> HMSQSNRELVVDFLSYKLSQKGYSWSQFSDVEENRTEAPEETEAERETPSAINGNPSWHLADSPAVNGATGHSSSLDAREVIPMAAVKQALREAGDEFELRARRAFSDLTSQ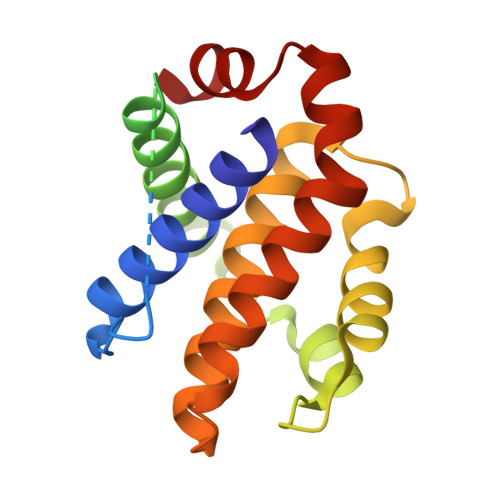LHITPGTAYQSFEQVVNELFRDGVNWGRIVAFFSFGGALCVESVDKEMQVLVSRIASWMATYLNDHLEPWIQENGGWDTFVDLYG>[2x]MEGSLLASGALLGADELARYFPDRNVALFVATWNMQGQKELPPSLDEFLLPAEADYAQDLYVIGVQEGCSDRREWETRLQETLGPHYVLLSSAAHGVLYMSLFIRRDLIWFCSEVECSTVTTRIVSQIKTKGALGISFTFFGTSFLFITSHFTSGDGKVAERLLDYTRTVQALVLPRNVPDTNPYRSSAADV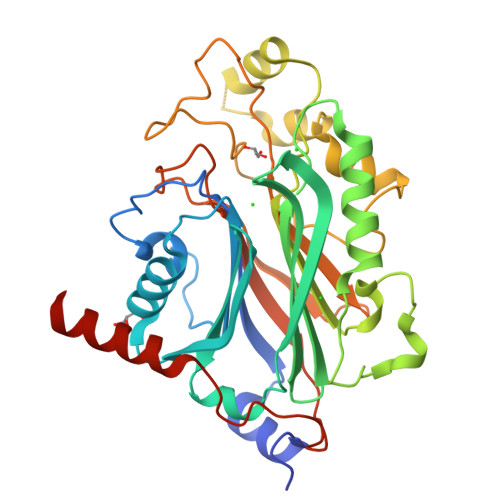TTRFDEVFWFGDFNFRLSGGRTVVDALLCQGLVVDVPALLQHDQLIREMRKGSIFKGFQEPDIHFLPSYKFDIGKDTYDSTSKQRTPSYTDRVLYRSRHKGDICPVSYSSCPGIKTSDHRPVYGLFRVKVRPGRDNIPLAAGKFDRELYLLGIKRRISAHHHHHH N-heptyl-N~3~-[(2R)-2-hydroxy-3,3-dimethyl-4-(phosphonooxy)butanoyl]-beta-alaninamide | C16 H33 N2 O7 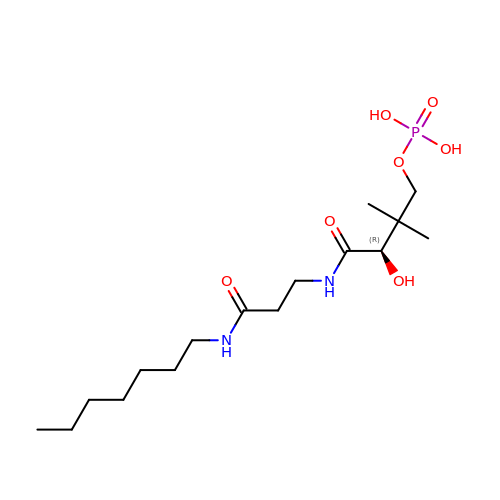P | QTSWMJJVYAHWSJ-AWEZNQCLSA-N>[4x]MTGGMKPPARKPRILNSDGSSNITRLGLEKRGWLDDHYHDLLTVSWPVFITLITGLYLVTNALFALAYLACGDVIENARPGSFTD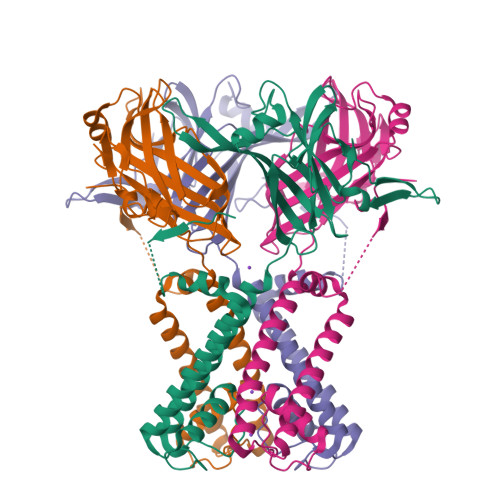AFFFSVQTMATIGYGKLIPIGPLANTLVTLEALCGMLGLAVAASLIYARFTRPTAGVLFSSRMVISDFEGKPTLMMRLANLRIEQIIEADVHLVLVRSEISQEGMVFRRFHDLTLTRSRSPIFSLSWTVMHPIDHHSPIYGETDETLRNSHSEFLVLFTGHHEAFAQNVHARHAYSCDEIIWGGHFVDVFTTLPDGRRALDLGKFHEIAQHHHHHH> TAA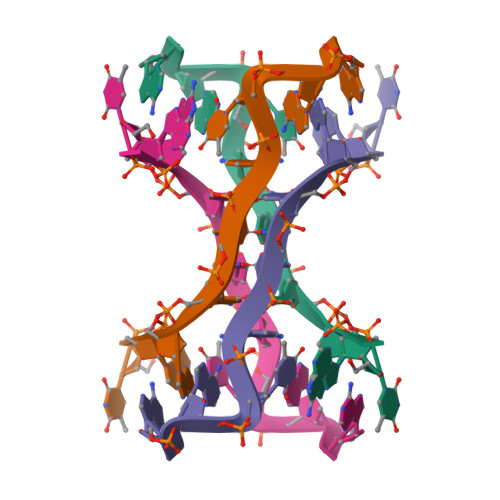CCCTAA>[6x]GAMDPMYLLVDVGNTHSVFSITEDGKTFRRWRLSTGVFQTEDELFSHLHPLLGDAMREIKGIGVASVVPTQNTVIERFSQKYFHISPIWVKAKNGCVKWNVKNPSEVGADRVANVVAFVKEYGKNGIIIDMGTATTVDLVVNGSYEGGAILPGFFMMVHSLFRGTAKLPLVEVKPADFVVGKDTEENIRLGVVNGSVYALEGIIGRIKEVYGDLPVVLTGGQSKIVKDMIKHEIFD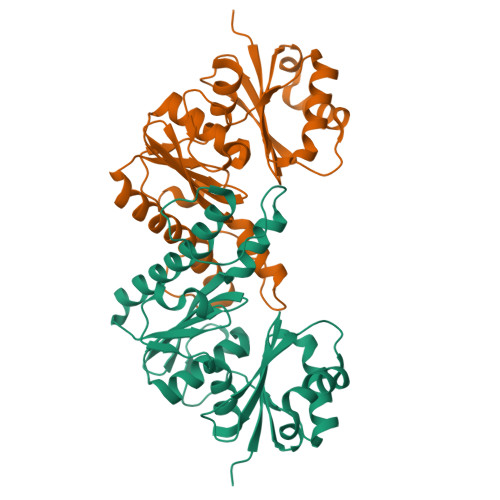EDLTIKGVYHFCFGD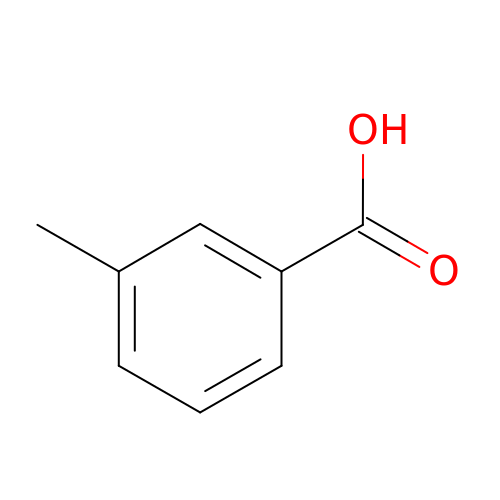3-methylbenzoic acid | C8 H8 O2 | GPSDUZXPYCFOSQ-UHFFFAOYSA-N> MENGYTYEDYKNTAEWLLSHTKHRPQVAIICGSGLGGLTDKLTQAQIFDYSEIPNFPRSTVPGHAGRLVFGFLNGRACVMMQGRFHMYEGYPLWKVTFPVRVFHLLGVDTLVVTNAAGGLNPKFEVGDIMLIRDHINLPGFSGQNPLRGPNDERFGDRFPAMSDAYDRTMRQRALSTWKQMGEQRELQEGTYVMVAGPSFETVAECRVL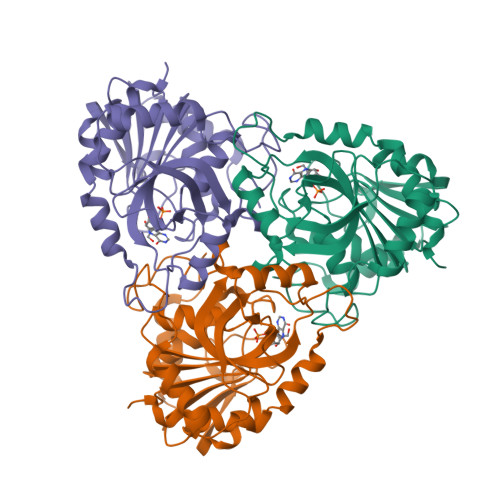QKLGADAVGMSTVPEVIVARHCGLRVFGFSLITNKVIMDYESLEKANHEEVLAAGKQAAQKLEQFVSILMASIPLPDKAS>[2x]MGSSHHHHHHSSGLEVLFQGPAMATKKVHIISHSHWDREWYMAYEQHHMRLINLIDDLLEVFQTDPDFHSFHLDGQTIILDDYLKVRPEREPEIRQAIASGKLRIGPFYILQDDFLTSSESNVRNMLIGKEDCDRWGASVPLGYFPDTFGNMGQTPQLMLKAGLQAAAFGRGIRPTGFNNQVDTSEKYSSQFSEISWQGPDNSRILGLLFANWYSNGNEIPTTEAEARLFWDKKLADAERFASTKHLLMMNGCDHQPVQLDVTKAIALANQLYPDYEFVHSCFEDYLADLADDLPENLSTVQGEITSQETD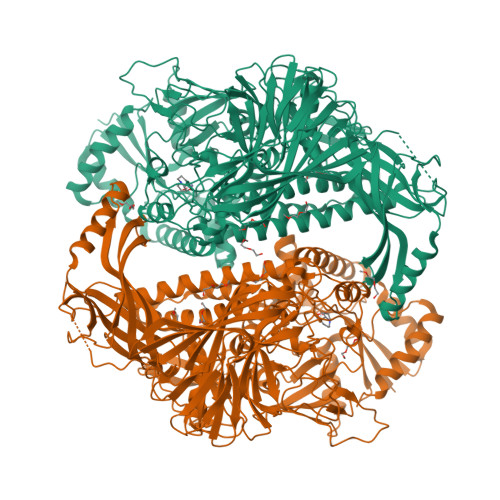GWYTLANTASARIYLKQANTRVSRQLENITEPLAAMAYEVTSTYPHDQLRYAWKTLMQNHPHDSICGCSVDSVHREMMTRFEKAYEVGHYLAKEAAKQIADAIDTRDFPMDSQPFVLFNTSGHSKTSVAELSLTWKKYHFGQRFPKEVYQEAQEYLARLSQSFQIIDTSGQVRPEAEILGTSIAFDYDLPKRSFREPYFAIKVRLRLPITLPAMSWKTLALKLGNETTPSETVSLYDDSNQCLENGFLKVMIQTDGRLTITDKQSGLIYQDLLRFEDCGDIGNEYISRQPNHDQPFYADQGTIKLNIISNTAQVAELEIQQTFAIPISADKLLQAEMEAVIDITERQARRSQEKAELTLTTLIRMEKNNPRLQFTTRFDNQMTNHRLRVLFPTHLKTDHHLADSIFETVKRPNHPDATFWKNPSNPQHQECFVSLFDGENGVTIGNYGLNEYEILPDTNTIAITLLRSVGEMGDWGYFPTPEAQCLGKHSLSYSFESITKQTQFASYWRAQEGQVPVITTQTNQHEGTLAAEYSYLTGTNDQVALTAFKRRLADNALITRSYNLSNDKTCDFSLSLPNYNAKVTNLLEKDSKQSTPSQLGKAEILTLAWKKQ> MGWSLPKEKGLILCLWNKFCRWFHRRESWAQSRDEQNLLQQKRIWESPLLLAAKENNVQALYKLLKFEGCEVHQKGAMGETALHIAALYDNNEAAQVLMEAAPELVFEPMTSELYEGQTALHIAVINQNVNLVRALLARGASVSARATGSVFHYRPHNLIYYGEHPLSFAACVGSEEIVRLLIEHGADIRAQDSLGNTVLHILILQPNKTFACQMYNLLLSYDGGDHLKSLELVPNNQGLTPFKLAGVEGNIVMFQHLMQKRKHIQWTYGPLTSTLYDLTEIDSSGDDQSLLELIVTTKKREARQILDQTPVKELVSLKWKRYGRPYFCVLGAIYVLYIICFTMCCVYRPLKPRITNRTNPRDNTLLQQKLLQEAYVTPKDDLRLVGELVSIVGAVIILLVEIPDIFRLGVTRFFGQTILGGPFHVIIVTYAFMVLVTMVMRLTNSDGEVVPMSFALVLGWCNVMAFARGFQMLGPFTIMIQKMIFGDLMRFCWLMAVVILGFASAFYIIFQTEDPDELGHFYDYPMALFSTFELFLTIIDGPANYDVDLPFMYSITYAAFAIIATL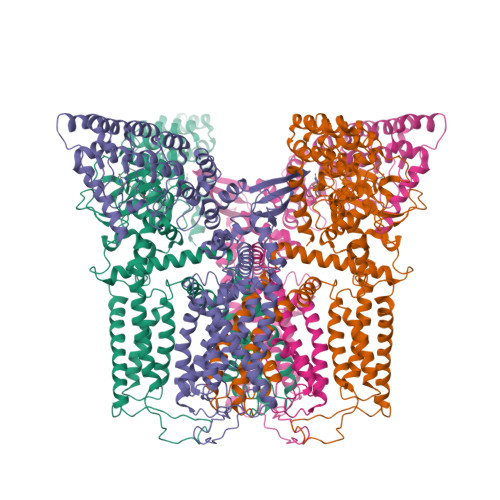LMLNLLIAMMGDTHWRVAHERDELWRAQVVATTVMLERKLPRCLWPRSGICGREYGLGDRWFLRVEDRQDLNRQRIRRYAQAFQQQDDLYSEDLEKDSGEKLVPR>VNVVAGGPVANYQIKVLDDGKIDKSATESPANNDVQLKVYAVDANGNIVGDITNDVTITSEATDTNGVIVNASKSTANGDTVYVITDNGSKKVGKETLTVKLGTVTLGTVDVEVIDTTLKATVVTKKADLIELDAADNGDALAKLLANLDIKDQ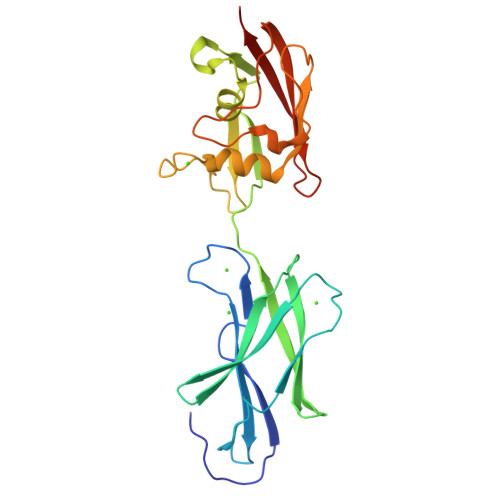NGNPMVDSAATPNTNEKLQALKSVLSGIVSSDTSVIGSVSNVDNLKDDASISGLAVKKAGTVTLTLVFNEDSKIAPIAITVKAPAAT[4x]>[24x]MAQPSAGETQASENITLSLLDRIIAEGRMAHDDSQQDYARDMLAEFATQVLDEGMAIDKDTVSMINDRIAQIDALIGAQLDEILHHPELQKLEASWRGLHMLVKNTETGARLKLRLLNVTQKELLIDLEKAVEFDQSALFKKIYEEEYGTFGGHPFSLLVGDYSFGRHPQDIGLLEKLSNVAAAAHAPFIAAASPRLFDMGSFTELAVPRDLAKIFESQELIKWRAFRESEDSRYVSLVLPHVLLRLPYGPDTCPVEGMDYVEDVNGRDHARYLWGNAA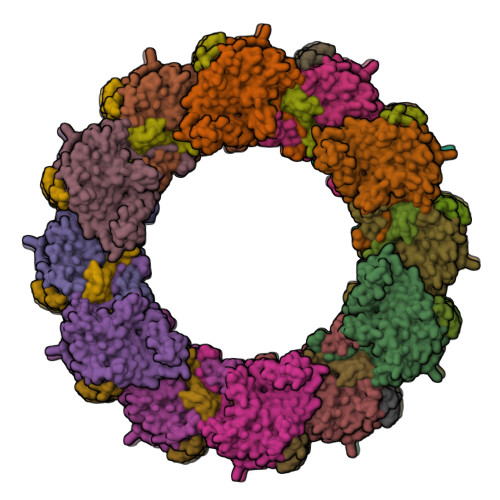WALTQRITEAFARYGWCAAIRGVEGGGAVEGLPAHSFRTSSGDLSLKCPTEVAITDRREKELDALGFIALCHKKNSDLAVFFGSQTTNRPRVYNTNEANANARISAMLPYVLAASRFAHYLKVIMRDKVGSFMTRDNVQTYLNNWIADYVLINDNAPQEIKAQYPLREARVDVSEVVGKPGVYRATVFLRPHFQLEELTASIRLVATLPPPAAA;>[24x]MAESTQHKLDRIRPPRVQITYDVETGNAIEKKELPLVVGILADLSGKPEKPLPKLMERRFVEINRDNFNDVLASIAPRAALQVDNTLSQDGSKLNIELHFDHIDDFDPVNIVRQVTPLRRLFEARQRLRDLLTKLDGNDDLDKLLQDVVANTEGLQEIRSARPQAENPAGAPGAEPAADEPAAEPQA> MTGGTGADAASAGASSTRPELRGERCLPPAGPVKVTPDDPRYLNLKLRGANSRFNGEPDYIHLVGSTQQVADAVEETVRTGKRVAVRSGGHCFEDFVDNPDVKVIIDMSLLTEIAYDPSMNAFLIEPGNTLSEVYEKLYLGWNVTIPGGVCGGVGVGGHICGGGYGPLSRQFGSVVDYLYAVEVVVVNKQGKARVIVATRERDDPH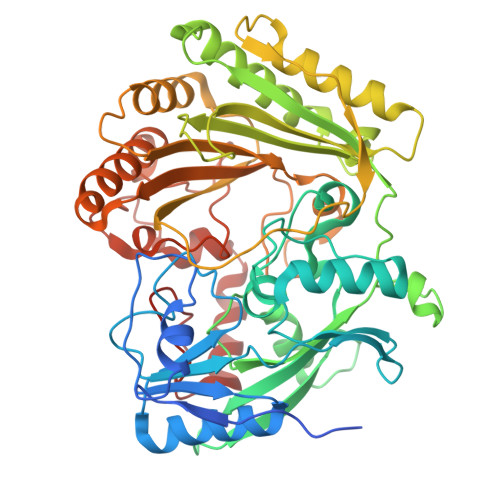HDLWWAHTGGGGGNFGVVTKYWMRVPEDVGRNPERLLPKPPATLLTSTVTFDWAGMTEAAFSRLLRNHGEWYERNSGPDSPYTGLWSQLMIGNEVPGMGESGFMMPIQVDATRPDARRLLDAHIEAVIDGVPPAEVPEPIEQRWLASTPGRGGRGPASKTKAGYLRKRLTDRQIQAVYENMTHMDGIDYGAVWLIGYGGKVNTVDPAATALPQRDAILKVNYITGWANPGNEAKHLTWVRKLYADVYAETGGVPVPNDVSDGAYINYPDSDLADPGLNTSGVPWHDLYYKGNHPRLRKVKAAYDPRNHFHHALSIRP> MANCRILLTPLNERDEQRGYSTQGLKRLSGTAKLNPRLGFTRTQFVQELPRQQKGMAISGYQPK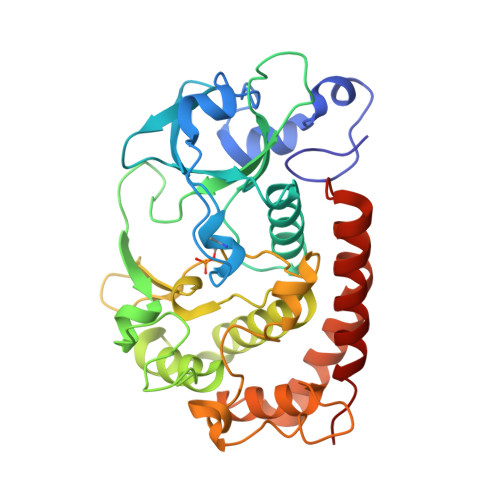LQLVLDEGEFRVVDHQGNFILKPSPADFPGLAENEHATMTLMSRLGFDVPVHGLLSFAPQSEEELEYAFVIRRYDRDNKGLPVHQEQLDGAMQITDKYGKTGNDNEQYVSYETLARFLVAHVNDNIAFKIDLFRRIVYAWLLGNNDMHLRNFGLVYSDGLTPALAPVYDFVSVAPYPEYFYSNYLALPLLTREEGGRELAPGFHSDYGEYIGQDFLLLGESMGLAPRLLEKLFQDIRKENAIVMETYEQSFMTQDHIQAVLQCYRHRLGLLHHHHHH>[6x]MTNTDLKPLLDNLRNATEFWNLVAAASATDESTVHNRSYRDALDWL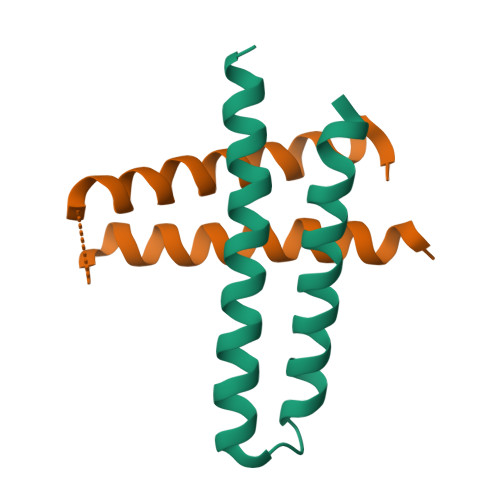ESAALALGDALIAQRKAVGGDHE> MGSADASTFLNRVCGVSAARLTPCGTGTSTDVVYRAFDIYNEKVAGFAKFLKTNCCRFQEKDEEGNLLDSYFVVKRHTMSNYQHEETIYNLVKDCPAVAVHDFFKFRVDGDMVPHISRQRLTKYTMADLVYALRHFDEGNCDTLKEILVTYNCCDDDYFNKKDWYDFVENPDILRVYANLGERVRQSLLKTVQFCDAMRDAGIVGVLTLDNQDLNGNWYDFGDFVQVAPGCGVPIVDSYYSLLMPILTLTRALAAESHMDADLAKPLIKWDLLKYDFTEERLCLFDRYFKYWDQTYHPNCINCLDDRCILHCANFNVLFSTVFPPTSFGPLVRKIFVDGVPFVVSTGYHFRELGVVHNQDVNLHSSRLSFKELLVYAADPAMHAASGNLLLDKRTTCFSVAALTNNVAFQTVKPGNFNKDFYDFAVSKGFFKEGSSVELKHFFFAQDGNAAISDYDYYRYNLPTMCDIRQLLFVVEVVDKYFDCYDGGCINANQVIVNNLDKSAGFPFNKWGKARLYYDSMSYEDQDALFAYTKRNVIPTITQMNLKYAISAKNRARTVAGVSICSTMTNRQFHQKLLKSIAATRGATVVIGTSKFYGGWHNMLKTVYSDVETPHLMGWDYPKCDRAMPNMLRIMASLVLARKHNTCCNLSHRFYRLANECAQVLSEMVMCGGSLYVKPGGTSSGDATTAYANSVFNICQAVTANVNALLSTDGNKIADKY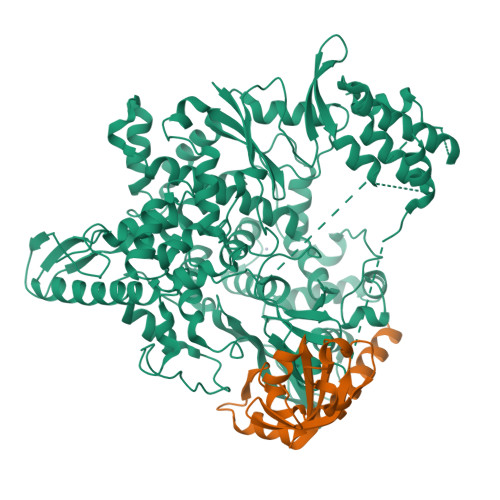VRNLQHRLYECLYRNRDVDHEFVDEFYAYLRKHFSMMILSDDAVVCYNSNYAAQGLVASIKNFKAVLYYQNNVFMSEAKCWTETDLTKGPHEFCSQHTMLVKQGDDYVYLPYPDPSRILGAGCFVDDIVKTDGTLMIERFVSLAIDAYPLTKHPNQEYADVFHLYLQYIRKLHDELTGHMLDMYSVMLTNDNTSRYWEPEFYEAMYTPHTVLLVPRGSGHHHHHHAWSHPQFEK;> AIASEFSSLPSYAAYATAQEAYEQAVANGDSEVVLKKLKKSLNVAKSEFDRDAAMQRKLEKMADQAMTQMYKQARSEDKRAKVTSAMQTMLFTMLRKLDNDALNNIINNARDGCVPLNIIPLTTAAKLMVVVPDYGTYKNTCDGNTFTYASALWEIQQVVDADSKIVQLSEINMDNSPNLAWPLIVTALRANSAVKLQ> ELSENFKKLMKYPY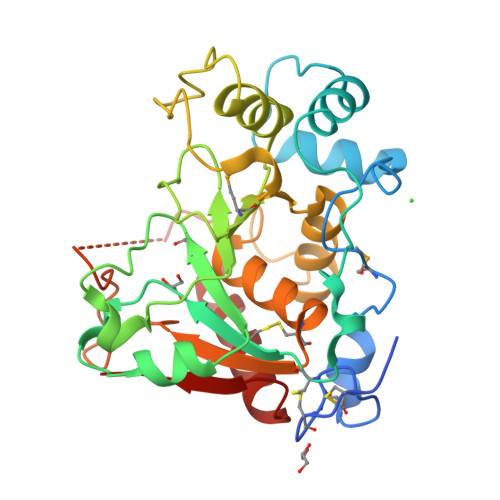RPCTCTRCIEEQRVSAWFDERFNRSMQPLLTAKNAHLEEDTYKWWLRLQREKKPNNLNDTIRELFQVVPGNVDPLLEKRLVSCRRCAVVGNSGNLKESYYGPQIDSHDFVLRMNKAPTEGFEADVGSKTTHHFVYPESFRELAQEVSMILVPFKTTDLEWVISATTTGRISHTYVPVPAKIKVKKEKILIYHPAFIKYVFDRWLQGHGRYPSTGILSVIFSLHICDEVDLYGFGADSKGNWHHYWENNPSAGAFRKTGVHDGDFESNVTTILASINKIRIFKGR> FHASTEAVRR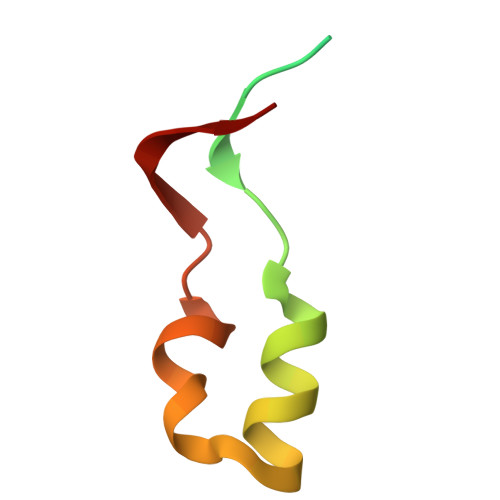VLPTEVTHIDARFNVSRVAVMIVALQQRPDLLWEGTRDRLHQPYR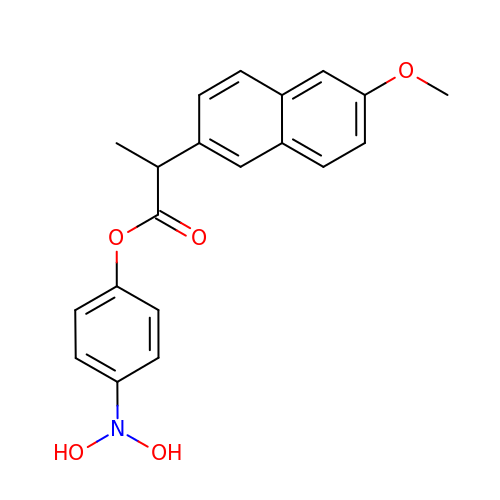(4-nitrophenyl) (2~{S})-2-(6-methoxynaphthalen-2-yl)propanoate | C20 H19 N O5 | DDQGDHCOPRIKDU-ZDUSSCGKSA-N> MKDRTQELRTAKDSDDDDDVTVTVDRDRFMDEFFEQVEEIRGFIDKIAENVEEVKRKHSAILASPNPDEKTKEELEELMSDIKKTANKVRSKLKSIEQSIEQEEGLNRSSADLRIRKTQHSTLSRKFVEVMSEYNATQSDYRERCKGRIQRQLEITGRTTTSEE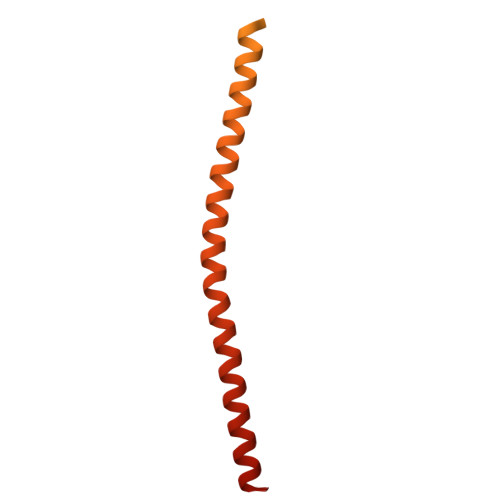LEDMLESGNPAIFASGIIMDSSISKQALSEIETRHSEIIKLENSIRELHDMFMDMAMLVESQGEMIDRIEYNVEHAVDYVERAVSDTKKAVKYQSKARRKKIM>[3x]GPHMGGSMSSALSQASPTAPRFSVLSWPQVRRLDAILCESVPIHGRGNFPTLSCRPRDLVQVVRSRLEQKGILVHNVRLNGSAASYVLHHDSGLGYKDLDLIFMVDLKGPDAFQVVKHAVLNCLLDFLPSGVNKEKITPMTLKEAYVQKLVKVCTESDRWSLISLSNNSGKNMELKFVDSLRRQFEFSVDSFQIILDSMLMFSQCSENPMSQSFHPTVTGESMYGDFEEAMDHLRNRI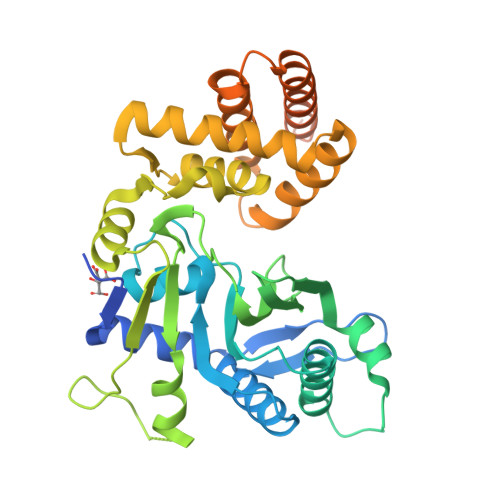IATRNPEEIRGGGLLKYCNLLVRGFRPKSEVDMKTMQRYMCSRYFIDFPDIREQQRKLKCYLQDHFVGMEDKRYDYLMTLHQVVNESTVCLMGHERRQTLALIASLAVHVLSEQNHPQAVPTFTCYYQPAPYIGEVNYNSYYFTPVQPLMSCSHSYQTWLPCCN> GGSMATVTATTKVPEIRDVTRIERIGAHSHIRGLGLDDALEPRQASQGMVGQLAARRAAGVVLEMIREGKIAGRAVLIAGQPGTGKTAIAMGMAQALGPDTPFTAIAGSEIFSLEMSKTEALTQAFRRSIGVRIKEGPPGVVHTVSLHEIDVINSRTQGFLALFSGDTGEIKSEVREQINAKVAEWREEGKAEIIPGVLFIDEVHMLDIESFSFLNRALESDMAPVLIMATNRGITRIRGTSYQSPHGIPIDLLDRLLIVSTTPYSEKDTKQILRIRCEEEDVEMSEDAYTVLTRIGLETSLRYAIQLITAASLVCRKRKGTEVQVDDIKRVYSLFLDESRSTQYMKEYQDAFLFNE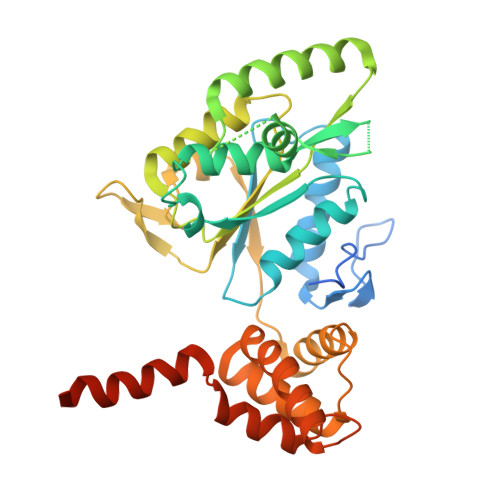LKGETMDTS The structural studies herein confirmed SAV0551 from S. aureus Mu50 as a member of the DJ-1 superfamily and that it has all the pertinent traits of this group, including the sandwich fold and nucleophilic arm. It specifically belongs to the Hsp-type subfamily because of the presence of cap domain and aspects of its dimeric interface. The results demonstrate that SAV0551 is a glyoxalase III that produces non-toxic D-lactate from toxic methylglyoxal independent of any cofactors. SAV0551 shows chaperone activity regardless of active site mutations, whereas the catalytic cysteine and active site residues are crucial for its glyoxalase III function.

To secure the SAV0551 glyoxalase III reaction intermediate and to determine the difference in the histidine location between A. thaliana DJ-1 and SAV0551, SAV0551 was crystallized with the DJ-1 glyoxalase III inhibitor glyoxylate. However, the glyoxylate in the SAV0551 crystal structure is not perfectly co-ordinated, potentially because of the relatively low resolution. Still, the SAV0551 co-crystal structure shows the clear density of the glyoxylate C1 and the interaction with Glu81 and Gly159. Amongst the three glyoxylate oxygen atoms, O3C2 does not form hydrogen bonds, while O1C1 and O2C2 show stable hydrogen bonds. O1C1 forms a hydrogen bond with His191 (2.93 Å) and Gly159 (2.48 Å). The C2 carbon–oxygen atom (O2C2) forms a hydrogen bond with His78 (2.83 Å) and a water molecule (2.71 Å). The third oxygen atom (O3C2) is 3.35 Å from a water molecule and 3.65 Å from His191, which demonstrate weak electrostatic bonds. The glyoxylate-bound crystal structure in SAV0551 is similar to the glyoxalase III reaction intermediate (hemithioacetal) because the glyxalase III substrate methylglyoxal has a single oxygen atom on C2. From the glyoxylate-bound structure, we determined that His78 provides a hydrogen atom to the O2C2 and that a water molecule attacks the C1 atom to hydrolyze the D-lactoylcysteine structure to produce D-lactate. Additionally, in the SAV0551 co-crystal structure, excess amounts of glyoxylate are also located in the aspartate-rich regions within the adjacent cleft of two irrelevant chains, which are not dimers.

>[8x]MSQDVNELSKQPTPDKAEDNAFFPSPYSLSQYTAPKTDFDGVEHKGAYKDGKWKVLMIAAEERYVLLENGKMFSTGNHPVEMLLPLHHLMEAGFDVDVATLSGYPVKLELWAMPTEDEAVISTYNKLKEKLKQPKKLADVIKNELGPDSDYLSVFIPGGHAAVVGISESEDVQQTLDWALDNDRFIVTLXHGPAALLSAGLNREKSPLEGYSVCVFPDSLDEGANIEIGYLPGRLKWLVADLLTKQGLKVVNDDMTGRTLKDRKLLTGDSPLASNELGKLAVNEMLNAIQNKLEHHHHHH> GSHMHERESSIRQLEA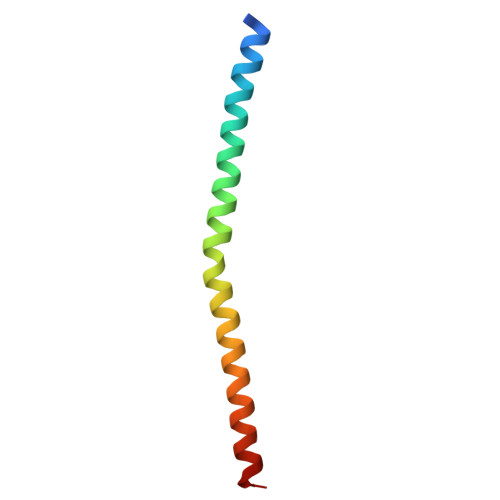DIMDINEIFKDLGMMIHEQGDVIDSIEANVESAEVHVQQANQQLSRAAN>[2x]MDKELGKTLRRLRQGKQVSISSLADEHLSKSQISRFERGESEISCSRLLNLLDKLNITIDEFVSTHSKTHTHFFTLLSRVRKYYAEKNVAKLLKLLEDYAHKDYESTMIKAILSSIEPTVEPSEEEVTRLTDYLFSVEQWGYYEIILLGNCSRFINYNT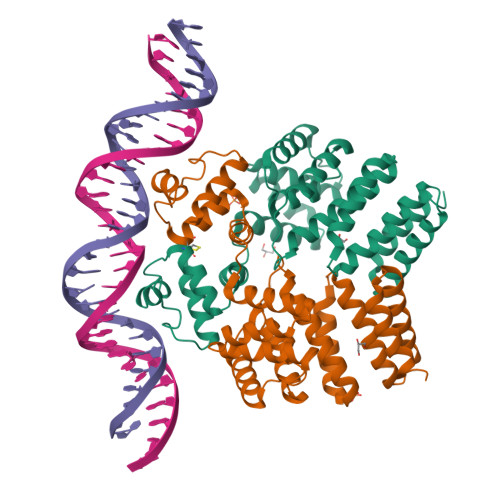LFLLTKEMVTSFAYSEQNKTNKTLVTQLSINCLIISIDYSYFDHSHYLIEKIEFLLRDELNFYEKTVFLYVHGYYKLKQGQVSGKDDMRQALQIFKYLGEDALYYSYKEHYRKEVLGDEEDEEEG The surfaces of most bacteria and archaea are covered with a proteinaceous coat, the surface or S-layer, which is formed through the self-assembly of individual protein subunits into a regularly spaced, two-dimensional array. In C. difficile, the S-layer largely consists of a major S-layer protein, SlpA, which assembles into a paracrystalline array enveloping the cell. The major protein of the C. difficile S-layer, SlpA, is post-translationally cleaved into two S-layer proteins (SLPs): the high molecular weight (HMW) and low molecular weight (LMW), herein referred to as SLPH and SLPL, respectively. These subunits then form a complex (referred to as H/L) that is incorporated in the S-layer.

Our H/L structural model reveals three distinct regions: a pseudo-threefold symmetric SLPH tile, an intricate LID/HID interacting motif and a third region composed of two domains, D1 and D2, of SLPL. These regions define two separate planes, with the SLPL spanning ~35 Å above the SLPH plane, linked by the LID/HID motif. SLPL protrudes from the interacting domains, with D1 closest to the SLPH plane and D2 extending outwards at an angle of ~120°, away from the long axis of D1. Conformational flexibility in the organisation of SlpA is further demonstrated by different arrangements observed in the structure of a truncated derivative of SlpA (SLPL/HID) and the H/L complex. The calculated rotation angle of the centres of mass of the D1-D2 region relative to LID/HID of 166° suggests a high degree of flexibility of these regions, at least in the absence of the CWB2-containing SLPH core, with minimal effects on the fold of each individual domain. The strikingly different arrangements of the D1-D2 domains in SLPL, relative to the interacting domains observed in the H/L and SLPL/HID structures, are consistent with this proposed flexibility.

>DSTTPGYTVVKNDWKKAVKQLQDGLKNKTISTIKVSFNGNSVGEVTPASSGAKKADRDAAAEKLYNLVNTQLDKLGDGDYVDFEVTYNLATQIITKAEAEAVLTKLQQYNDKVLINSATDTVKGMVSDTQVDSKNVAANPLKVSDMYTIPSAITGSDDSGYSIAKPTEKTTSLLYGTVGDATAGKAITVDTASNEAFAGNGKVIDYNKSFKATVQGDGTVKTSGVVLKDASDMAATGTIKVRVTSAKEESIDVDSSSYISAENLAKKYVFNPKEVSEAYNAIVALQNDGIESDLVQLVNGKYQVIFYPEGKRLETKS[2x];>[2x]ADIIADADSPAKITIKANKLKDLKDYVDDLKTYNNTYSNVVTVAGEDRIETAIELSSKYYNSDDKNAITDDAVNNIVLVGSTSIVDGLVASPLASEKTAPLLLTSKDKLDSSVKSEIKRVMNLKSDTGINTSKKVYLAGGVNSISKDVENELKNMGLKVTRLSGEDRYETSLAIADEIGLDNDKAFVVGGTGLADAMSIAPVASQLKDGDATPIVVVDGKAKEISDDAKSFLGTSDVDIIGGKNSVSKEIEESIDSATGKTPDRISGDDRQATNAEVLKEDDYFKDGEVVNYFVAKDGSTKEDQLVDALAAAPIAGRFKESPAPIILATDTLSSDQNVAVSKAVPKDGGTNLVQVGKGIASSVINKMKDLLDM> GPHMLEQCINPFTNLPHTPRYYDILKKRLQLPVWEYKDRFTDILVRHQSFVLVGETGSGKTTQIPQWCVEYMRSLPGPKRGVACTQPRRVAAMSVAQRVADEMDVMLGQEVGYSIRFEDCSSAKTILKYMTDGMLLREAMNDPLLERYGVIILDEAHERTLATDILMGVLKEVVRQRSDLKVIVMSATLDAGKFQIYFDNCPLLTIPGRTHPVEI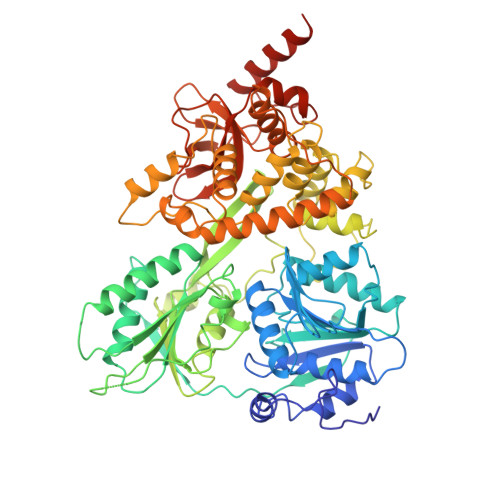FYTPEPERDYLEAAIRTVIQIHMCEEEEGDLLLFLTGQEEIDEACKRIKREVDDLGPEVGDIKIIPLYSTLPPQQQQRIFEPPPPKKQNGAIGRKVVVSTNIAETSLTIDGVVFVIDPGFAKQKVYNPRIRVESLLVTAISKASAQQRAGRAGRTRPGKCFRLYTEKAYKTEMQDNTYPEILRSNLGSVVLQLKKLGIDDLVHFDFMDPPAPETLMRALELLNYLAALNDDGDLTELGSMMAEFPLDPQLAKMVIASCDYNCSNEVLSITAMLSVPQCFVRPTEAKKAADEAKMRFAHIDGDHLTLLNVYHAFKQNHESVQWCYDNFINYRSLMSADNVRQQLSRIMDRFNLPRRSTDFTSRDYYINIRKALVTGYFMQVAHLERTGHYLTVKDNQVVQLHPSTVLDHKPEWVLYNEFVLTTKNYIRTCTDIKPEWLVKIAPQYYDMSNFPQCEAKRQLDRIIAKLQSKEYSQY> MFEARLVQGSILKKVLEALKDLINEACWDISSSGVNLQSMDSSHVSLVQLTLRSEGFDTYRCDRNLAMGVNLTSMSKILKCAGNEDIITLRAEDNADTLALVFEAPNQEKVSDYEMKLMDLDVEQLGIPEQEYSCVVKMPSGEFARICRDLSHIGDAVVISCAKDGVKFSASGELGNGNIKLSQTS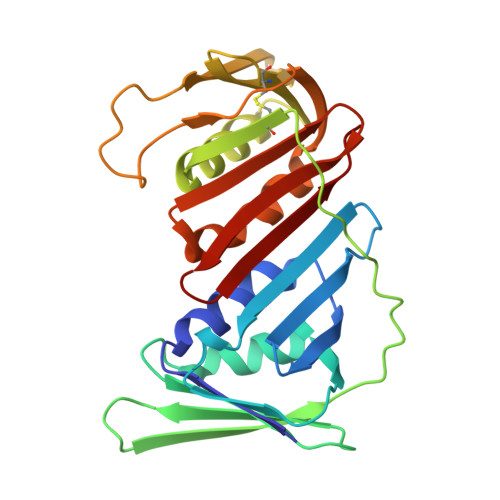NVDKEEEAVTIEMNEPVQLTFALRYLNFFTKATPLSSTVTLSMSADVPLVVEYKIADMGHLKYYLAPK>MGMLTEQPNWLMQRAQLTPERIALIYEDQTVTFAELFAASKRMAEQLAAHSVRKGDTAAILLQNRAEMVYAVHACFLLGVKAVLLNTKLSTHERLFQLEDSGSGFLLTDSSFEKKEYEHIVQTIDVDELMKEAAEEIEIEAYMQMDATATLMYTSGTTGKPKGVQQTFGNHYFSAVSSALNLGITEQDRWLIALPLFHISGLSALFKSVIYGMTVVLHQRFSVSDVLHSINRHEVTMISAVQTMLASLLEETNRCPESIRCILLGGGPAPLPLLEEC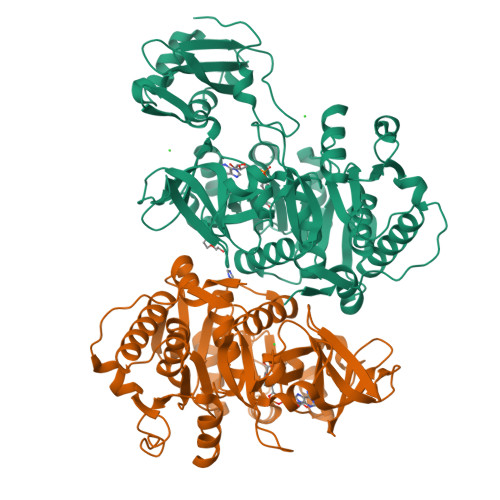REKGFPVFQSYGMTETCSQIVTLSPEFSMEKLGSAGKPLFSCEIKIERDGQVCEPYEHGEIMVKGPNVMKSYFNRESANEASFQNGWLKTGDLGYLDNEGFLYVLDRRSDLIISGGENIYPAEVESVLLSHPAVAEAGVSGAEDKKWGKVPHAYLVLHKPVSAGELTDYCKERLAKYKIPAKFFVLDRLPRNASNKLLRNQLKDARKGELLHHHHHH[2x]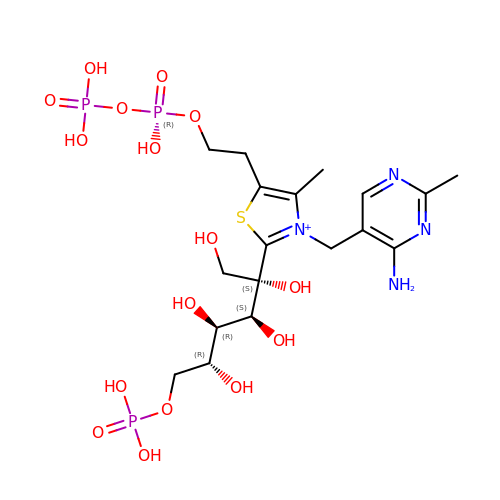2-C-{3-[(4-amino-2-methylpyrimidin-5-yl)methyl]-5-(2-{[(R)-hydroxy(phosphonooxy)phosphoryl]oxy}ethyl)-4-methyl-1,3-thiazol-3-ium-2-yl}-6-O-phosphono-D-glucitol | C18 H32 N4 O16 P3 S | AJFWOWNNZFXSES-TXPWEPMLSA-O>[2x]GSSGSSGIGEGMLADFVSQTSPMIPSIVVHCVNEIEQRGLTETGLYRIDGCDRTVKELKEKFLRVKTVPLLSKVDDIHAICSLLKDFLRNLKEPLLTFRLNRAFMEAAEITDEDNSIAAMY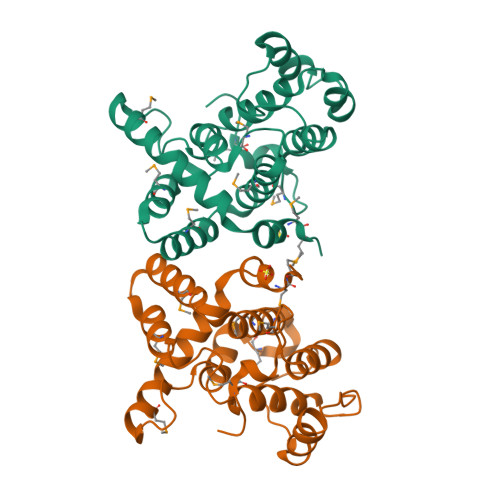QAVGELPQANRDTLAFLMIHLQRVAQSPHTKMDVANLAKVFGPTIVAHAVPNPDPVTMSQDIKRQPKVVERLLSLPLEYWSQFMMVE Retinoschisin, an octameric retinal-specific protein, is essential for retinal architecture with mutations causing X-linked retinoschisis (XLRS), a monogenic form of macular degeneration. Retinoschisin, a 24kDa protein secreted by photoreceptors, consists of a retinoschisin (Rs1) domain and a discoidin domain with a small C-terminal extension. Uniquely, the cysteine rich Rs1 domain and the C-terminal extension in retinoschisin mediate the formation of a C59-C223 disulfide linkage which is essential for octamerisation. Retinoschisin forms a dimer of octamers with each octameric ring adopting a planar propeller structure.

Previously, the disease-causing R141H mutation was found to be secreted as an octamer at similar levels to wild-type retinoschisin. R141H also formed octamer and dimer of octamer species, with imaging under cryo-EM conditions confirming a similar double-stack arrangement to the wild-type. Moreover, the increased number of side views allowed for 3D reconstruction of the R141H complex at the higher resolution of 4.2Å. This revealed a comparable domain arrangement to the wild-type protein. A homology model of the R141H discoidin domain was constructed and fitted to the map using DockEM. As previously observed, the central density represented the flexible N-terminal Rs1 domains which were masked out in the refinement procedure. Comparison of the R141H hexadecamer structure to the wild-type retinoschisin map filtered at 5Å with DockEM, revealed a highly similar structure. Mapping of the R141H mutation indicated that it was located in a spike region distinct from intra- and inter-octamer interfaces with an overall positive charge. Comparison of the intrinsic fluorescence of wild-type and R141H mutant retinoschisin showed increased fluorescence in the mutant despite the lack of gross conformational change, suggesting a small change in the spike regions. The disulfide-linkage between spikes 3 and 2 (10) could act to propagate a conformational change in spike 3 to spike 2, generating a wider subtle reorganization of the spikes at the propeller tips.

>[16x]STEDEGEDPWYQKACKCDCQGGPNALWSAGATSLDCIPECPYHKPLGFESGEVTPDQITCSNPEQYVGWYSSWTANKARLNSQGFGCAWLSKFQDSSQWLQIDLKEIKVISGILTQGHCDIDEWMTKYSVQYRTDERLNWIYYKDQTGNNRVFYGNSDRTSTVQNLLRPPIISRFIRLIPLGWHVRIAIRMELLECVSKCA>GGGSMEVVGDFEYSKRDLVGHGAFAVVFR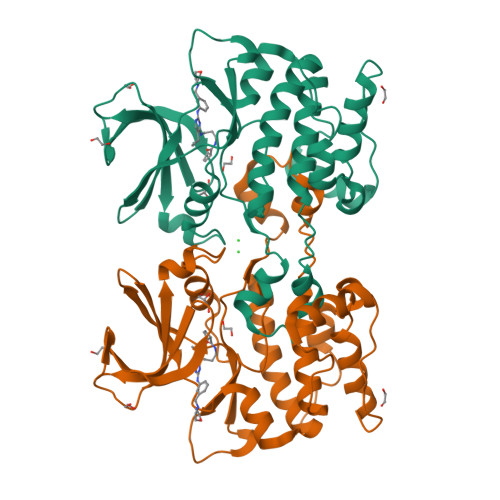GRHRQKTDWEVAIKSINKKNLSKSQILLGKEIKILKELQHENIVALYDVQELPNSVFLVMEYCNGGDLADYLQAKGTLSEDTIRVFLHQIAAAMRILHSKGIIHRDLKPQNILLSYANRRKSSVSGIRIKIADFGFARYLHSNMMAADLCGSPMYMAPEVIMSQHYDAKADLWSIGTVIYQCLVGKPPFQANSPQDLRMFYEKNRSLMPSIPRETSPYLANLLLGLLQRNQKDRMDFEAFFSHPFLEQGPV[3x]> SEGNGPAAVHYQPASPPRDACVYSSCYCEENVWKLCEYIKNHDQYPLEECYAVFISNERKMIPIWKQQARPGDGPVIWDYHVVLLHVSSGGQSFIYDLDTVLPFPCLFDTYVEDAIKSDDDIHPQFRRKFRVICADSYLKNFASDRSHMKDS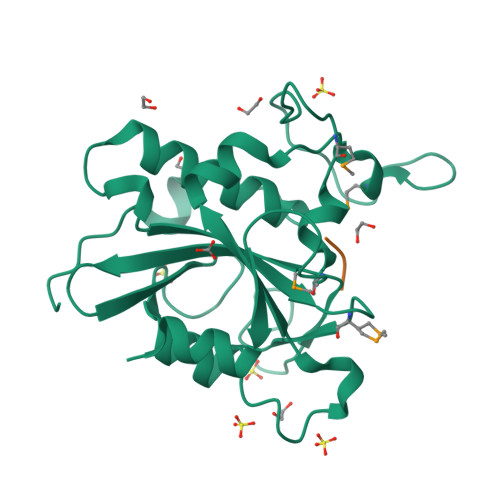SGNWREPPPPYPCIETGDSKMNLNDFISMDPKVGWGAVYTLSEFTHRFGSKNC;> STA>[2x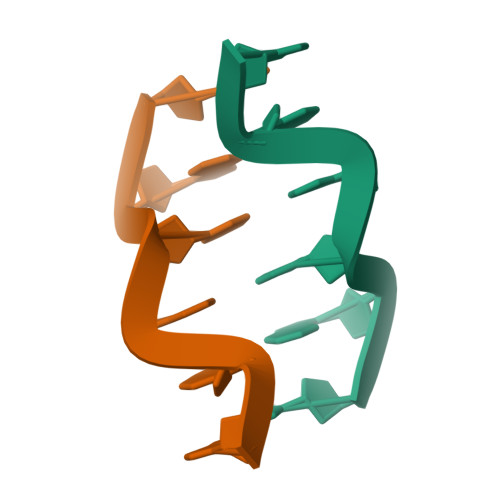]CGCGTG> HMLDPEEIRKRLEHTERQFRNRRKILIRGLPGDVTNQEVHDLLSDYELKYCFVDKYKGTAFVTLLNGEQAEAAINAFHQSRLRERELSVQLQPTDALLCVANLPPSLTQQQFEELVRPFGSLERCFLVYSERTGQSKGYGFAEYMKKDSAARAKSDLLGKPLGPRTLYVHWTDAGQLTPALLHSRCLCVDRLPPGFNDVDALCRALSAVHSPTFCQLACGQDGQLKGFAVLEYETAEMAEEAQQQADGLSLGGSHLRVSFCAPGPPGRSMLAALIAAQATALNR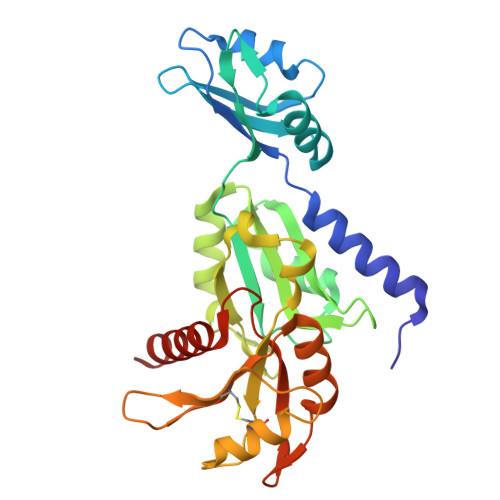G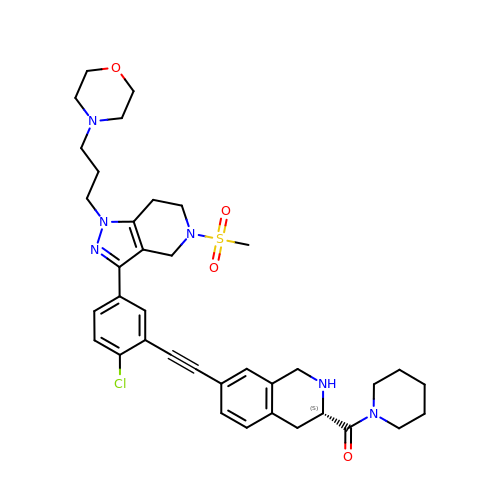{(3S)-7-[(2-chloro-5-{5-(methylsulfonyl)-1-[3-(morpholin-4-yl)propyl]-4,5,6,7-tetrahydro-1H-pyrazolo[4,3-c]pyridin-3-yl}phenyl)ethynyl]-1,2,3,4-tetrahydroisoquinolin-3-yl}(piperidin-1-yl)methanone | C37 H45 Cl N6 O4 S | BIYANWMTXPESQI-UMSFTDKQSA-N>[6x]MYINNGRINYNNEYGYRRGIYREPFYSDNADYNTNSKSYYDYLARFNGFIFELCDFVNGLADDIQKMKDTYEALTLSNTDVTYTVGQKGDFDTLNHCFEHIEDLIVQPKSIRVILLKDYMMREQLFLRDKRYNHITITSENDIVEAYETELNRQVEIKTNPIFRVKPLFYGINSTFPKIDFKLQNKDFSDTINCGFLMDNTTFEMTERGGSTHFNFIGLCGVNGSHIQTNYCDFSYNGNREQLEEYNKDQNMYGDGLRIFNSSLTGNYMTVNRCGEIGIHFSHGASGYIDFTEARFNGHHGLMVTTGSQASARNCKITDTIDDNVVSYASSDIDLRSSDCSNSQTTYGVIATRSSNINFDKGIANGCGASGIMANRGCSIDATGATASRNKWHGVIASNNSKVDFTSG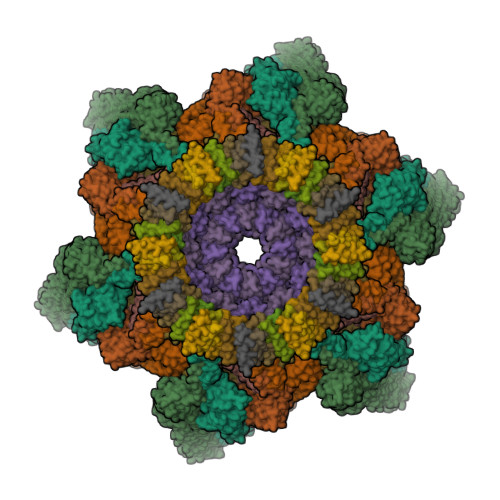NANENGLDGIQCTHGSTVQARLSTTNGNKRNGVLAYAGDVYCQEINCDGNGRRGLEATRGGYVAAYGAKVSRSKDDNVLAYGSMISINEALIERAGRNGIEATRGGQIFADRITITGSGDFGILAYASKVFAEASNISGTKNEPVYATRGGEVTCFGSNISSNKTVYNVYNGSRIFTDKDHGYSTNVDPQTLSSKGLIILG;>[2x]MSYLDNDYIGKNKDVGLKVELTEDIDRRIMEHRNRFRRLIFNRYVEFLPLLINYTNQNSVGIDFLQLEIALRQGYQVVVGKARNGVIMILGYIQSMYYKNSNDFINNFNLTFNKRLTQDDITFIIPDYLRPDYALEIEYYDNCQSGDFIVLRNKPVNLNNDYQIIEHYCDELAEIILSRFSLIMQSKFSKIFLSDIQDETINQFINKLYNGAPFIKTDKYIDPEEDIIDLGSDFVTTALVEMKREYQNKVSELSNFLGVNSLAVDKESGVSDTEAKSNRSFTTSNSNIYLRGRNPFEMLNRRFNLDIHPYYDDEAISEMDIMNLKTDNFGGGKVE;>LSKHTTTLYEIIESELQRLGLNEFVNNDRIHFNDSKHAFMQKMLYFDDDVKQIVDHMFFKGFMFNDERIDRYFKESFTLRFLYREIGRQTVESFASQVLYITMTHEDYIYRVYGSDMYKYIEQVTDTQSQDLGKAIENAIEQGQTKDRQQDKGHEEYKDYEDTITKSFDDNRTAESTLPQSKVNIDVDNTVLDYADTNTISRDKNTSETVSEKTGTKDNTFDSLRNGESDTKRNTQSQNEMNRTGLTKQYLIDNLQKLYSMRDTIFKTYDKECFLHIW[2x];>LIIKHQMKLHLNELVDWAWRNGVTSEKFHSNNGSYVIFDHSAVVETYIINKNDLFNVTEEIEITLDKPIDYFLEKDMYGNYREHFGIAINDLLFLNTTVNIWLVNDDNSHILIYKDGKLIDEYMYHQFEYEANQNKHIYPNNKASGTYPHKTEQDVTPPKKQPDTKPLPPEEHTPKVRTIKTLNGTVMKDYTPVSSIQYVKSVGIIGDSVGKGAHASYNFGDYINEKTGAKIQNLSVSSATMSEVKDNNILNQAKQLKDNELVIIQGTDDDWLFNSNAGVEVGNKITDTKTYIGAFYKVVETVKENNPKAKIVVITPTKQAKIDDTGKVIRRDTDKNKKGYTLKTYVDSQVKATKDLGLALYNAYDDSLINPYDEKFRQSSMKDGLHPTKWGHEMMYYRIAETYHKNFD[2x];>[12x]MAEEEKIIKEEPTNEETEQPEKIESAEDVVTEPEKEVTEEKSEAFVQLEQRISSLEQRLNNLESQPQPTQESSDPNFEDKTVPTEVDDNQETDGIESSEEIKQMLNL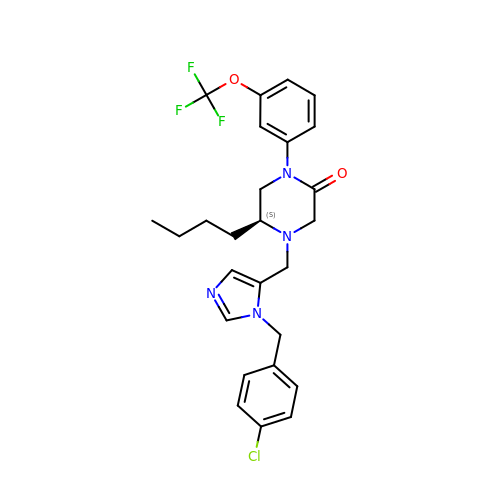(5S)-5-butyl-4-({1-[(4-chlorophenyl)methyl]-1H-imidazol-5-yl}methyl)-1-[3-(trifluoromethoxy)phenyl]piperazin-2-one | C26 H28 Cl F3 N4 O2 | POBHWQSJZMJUAH-QFIPXVFZSA-N>GAMASQLETAKEPCMAKFGPLPSKWQMASSEPPCVNKVSDWKLEILQNGLYLIYGQVAPNANYNDVAPFEVRLYKNKDMIQTLTNKSKIQNVGGTYELHV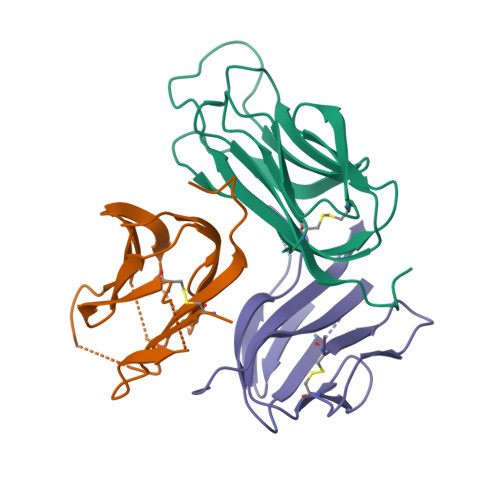GDTIDLIFNSEHQVLKNNTYWGIILLANPQFIS[3x]(3~{S},4~{R})-4,5,5-tris(oxidanyl)piperidine-3-carboxylic 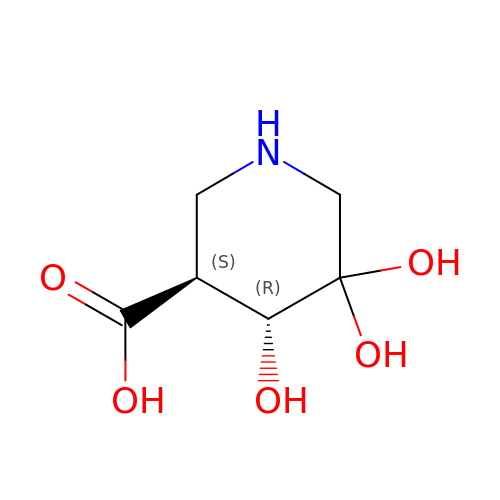acid | C6 H11 N O5 | VJJFPBNJYGLWRR-IUYQGCFVSA-N> GSAEYVRALFDFNGNDEEDLPFK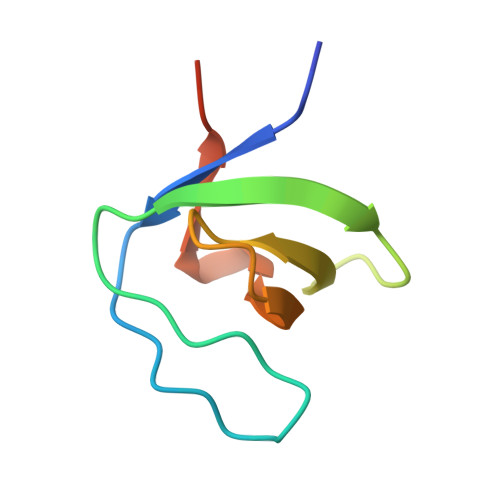KGDILRIRDKPEEQWWNAEDSEGKRGMIPVPYVEKYHHHHHH> M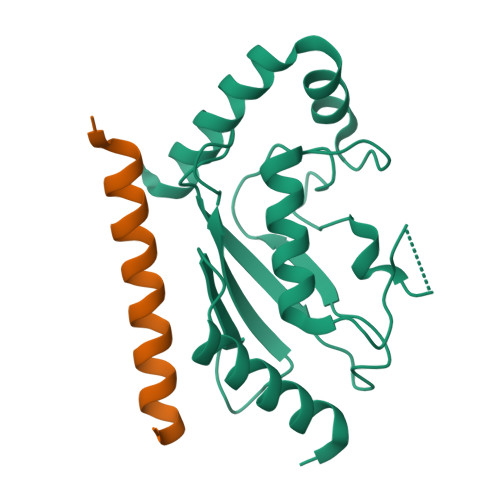AGTALKRLMAEYKQLTLNPPEGIVAGPMNEENFFEWEALIMGPEDTCFEFGVFPAILSFPLDYPLSPPKMRFTCEMFHPNIYPDGRVCISILHAPGDDPMGYESSAERWSPVQSVEKILLSVVSMLAEPNDESGANVDASKMWRDDREQFYKIAKQIVQKSLGL;> GPSWARQESLQERKQALYEYARRRFTERRAQEAD> IVGGYTCQENSVPYQVSLNSGYHFCGGSLINDQWVVSAAHCYKSRIQVRLGEHNINVLEGNEQFVNAAKIIKHPNFDRKTLNNDIMLIKLSSPVKLNARVATVALPSSCAPAGTQCLISGWGNTLSSGVNEPDLLQCLDAPLLPQADCEASYPGKITDNMVCVGFLEGGKGSCQGDSGGPVVCNGELQGIVSWGYGCALPDNPDVYTKVCNYVDWIQDTIAAN;> VREVCSEQAETGPCRAMISRW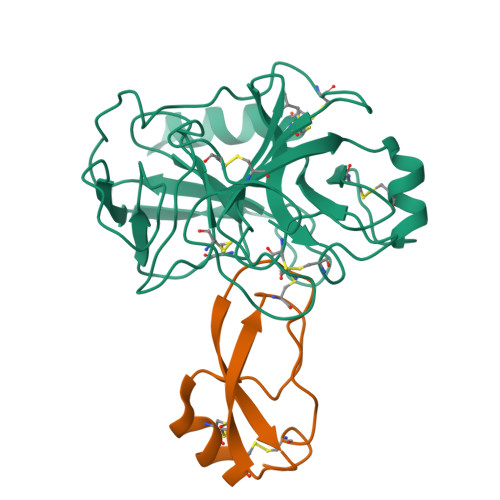YFDVTEGKCAPFFYGGCGGNRNNFDTEEYCMAVCG>GPLGSPTYHSFFVYCKGPCHKVQPGKLRVQCGTCRQATLTLAQGPSC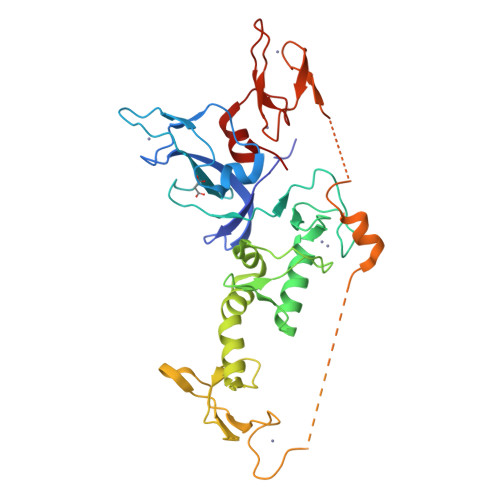WDDVLIPNRMSGECQSPDCPGTRAEFFFKCGAHPTSDKDTSVALNLITNNSRSIPCIACTDVRNPVLVFQCNHRHVICLDCFHLYCVTRLNDRQFVHDAQLGYSLPCVAGCPNSLIKELHHFRILGEEQYNRYQQYGAEECVLQMGGVLCPRPGCGAGLLPEQGQRKVTCEGGNGLGCGFVFCRDCKEAYHEGECDSMFEASGATSQAYRVDQRAAEQARWEEASKETIKKTTKPCPRCNVPIEKNGGCMHMKCPQPQCKLEWCWNCGCEWNRACMGDHWFDV[3x]> MVVIANAHNEMIHDAVMDYYGKRMATCSSDKTIKIFEVEGETHKLIDTLTGHEGPVWRVDWAHPKFGTILASCSYDGKVMIWKEENGRWSQIAVHAVHSASVNSVQWAPHEYGPMLLVASSDGKVSVVEFKENGTT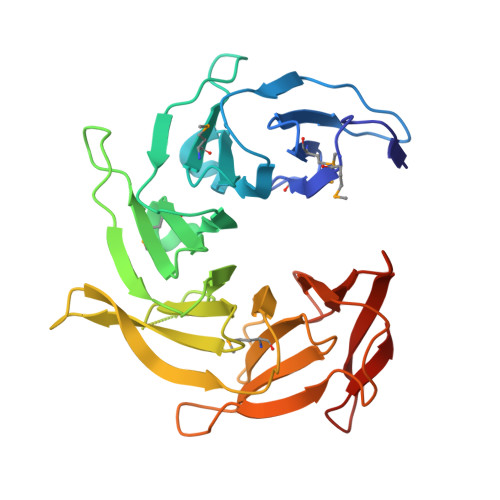SPIIIDAHAIGVNSASWAPATIEEDGEHNGTKESRKFVTGGADNLVKIWKYNSDAQTYVLESTLEGHSDWVRDVAWSPTVLLRSYMASVSQDRTCIIWTQDNEQGPWKKTLLKEEKFPDVLWRASWSLSGNVLALSGGDNKVTLWKENLEGKWEPAGEVHQ>QVVKPTDERIIDPSTANTQLTGGVCYNTTSGGNKPLAGSPYGYETWIDTGGGVCSLCWYGADQGGGAAFKATWTNPHDFLGRLGYFWNENKPYSHYENIYCGFNYTRSGRKTAGDYSYIGIYGWSRNPSASNSNERLIEYYIVEDWFGNQWQADTSPMGINTTGGTVMGSFTVDGSSYQIIKNTRVNQPSIEGDKTFVQYFSIRQSPRKSGT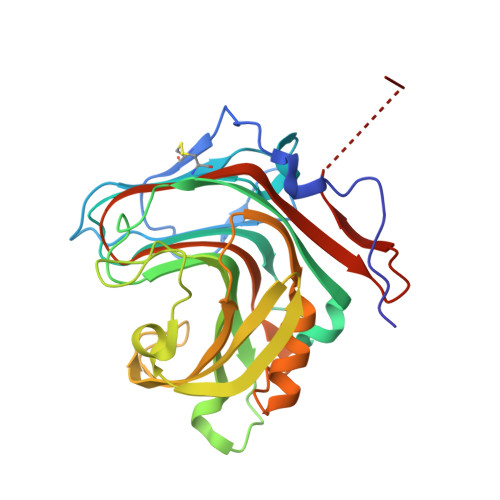ISITEHFKKWEKLGMKLGDNMYECKFLIEAGAGEGFFDARLIQFYRADNEGNILQITPLEHHHHHH[2x]> MTRSPRRPLFAVSLVLSAMLLAGAAHAAVSNEEILQDPKNPQQIVTNGLGVQGQRYSPLDLLNVNNVKELRPVWAFSFGGEKQRGQQAQPLIKDGVMYLTGSYSRVFAVDARTGKKLWQYDARLPDDIRPCCDVINRGVALYGNLVFFGTLDAKLVALNKDTGKVVWSKKVADHKEGYSISAAPMIVNGKLITGVAGGEFGVVGKIQAYNPENGELLWMRPTVEGHMGYVYKDGKAIENGISGGEAGKTWPGDLWKTGGAAPWLGGYYDPETNLILFGTGNPAPWNSHLRPGDNLYSSSRLALNPDDGTIKWHFQSTPHDGWDFDGVNELISFNYKDGGKEVKAAATADRNGFFYVLDRTNGKFIRGFPFVDKITWATGLDKDGRPIYNDASRPGAPGSEAKGSSVFVAPAVLGAKNWMPMAYNKDTGLFYVPSNEWGMDIWNEGIAYKKGAAFLGAGFTIKPLNEDYIGVLRAIDPVSGKEVWRHKNY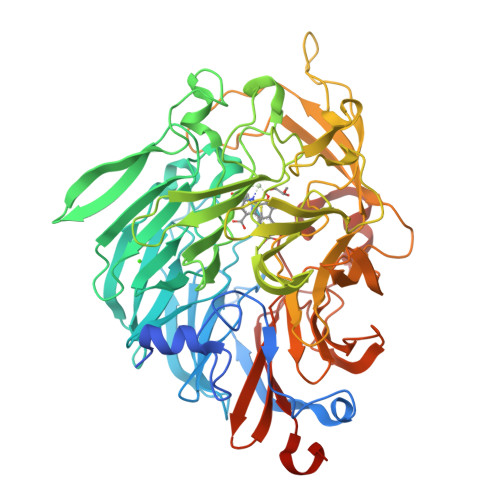APLWGGVLTTKGNLVFTGTPEGFLQAFNAKTGDKVWEFQTGSGVLGSPVTWEMDGEQYVSVVSGWGGAVPLAGGEVAKRVKDFNQGGMLWTFKLPKQLQQTASVKPHHHHHH KtrAB is a cation channel with a nucleotide-dependent RCK domain. The structure of the KtrAB complex revealed a homodimeric membrane protein (KtrB) assembled with a cytosolic RCK octameric ring, formed by the KtrA protein. KtrA binds nucleotides, ATP or ADP. ATP binding induces the adoption of a square-conformation by the octameric ring and increased K+ flux activity through KtrAB; ADP binding results in a non-square conformation and decreased flux.

A simple indicator of ring conformation is the pair of distances (L1 and L2) separating the Cα of N38 residues located in opposite subunits across a ring face. Like in the wild-type protein, the ADP-bound R16K (at 3.0 Å resolution) and R16A (at 3.7 Å resolution) rings adopt a non-square conformation. However, the ADP-bound ring conformations are different from each other and from the wild-type, with L1/L2 distances for the wild-type of 40.7/30.7 Å and for R16K of 52.0/21.9 Å. In contrast, we found a large structural variability in the non-square structures, with four different conformational groups based on Cα N38 L1/L2 distances. This indicates that there is a single well defined square or active conformation for KtrA, while the ring in the non-active (or non-square) conformation is most likely more flexible, giving rise to different ring conformations in the crystals of isolated KtrA.

>MGRIKNKQFAVIGLGKFGGSICKELHRMGHEVLAVDINEEKVNAYASYATHAVIANATEENELLSLGIRNFEYVIVAIGANIQASTLTTLLLKELDIPNIWVKAQNYYHHKVLEKIGADRIIHPEKDMGVKIAQSLSDENVLNYIDLSDEYSIVELLATRKLDSKSIIDLNVRAKYGCTILAIKHHGDICLSPAPEDIIREQDCLVIMGHKKDIKRFENEGM[8x]> SIITKSIVNADAEARYLSPGELDRIKSFVLSGQRRLRIAQILTDNRELIVKQGGQQLFQKRPDVVSPGGNAYGEEMTATCLRDLDYYLRLVTYGIVAGDVTPIEEIGLVGVKEMYNSLGTPISGVAEGVRSMKNVACSLLAGEDSAEAGFYFDYTLGAMQ;> MQDAITSVINAADVQGRYLDDNSLDKLRGYFQTGELRVRASATIAANAATIIKDSVA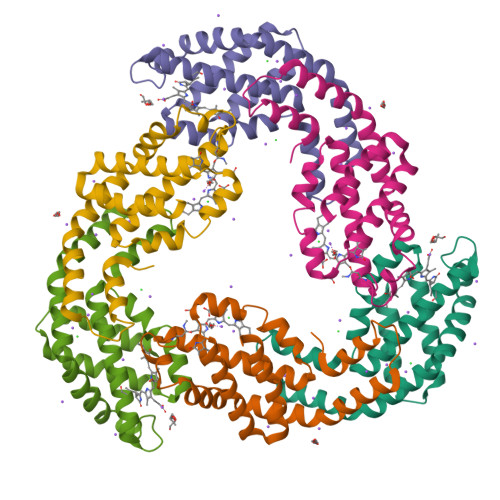KALLYSDITRPGGNMYTTRRYAACIRDLDYYLRYATYGMLAGDPSILDERVLNGLKETYNSLGVPIGATIQAVQAMKEVTSSLVGPDAGKEMGVYFDYICSGLS>GGSKPDCTAAMRDVRQQYESVAAKNLQEAEEWYKSKFADLSEAANRNNDALRQAKQESTEYRRQVQSLTMEV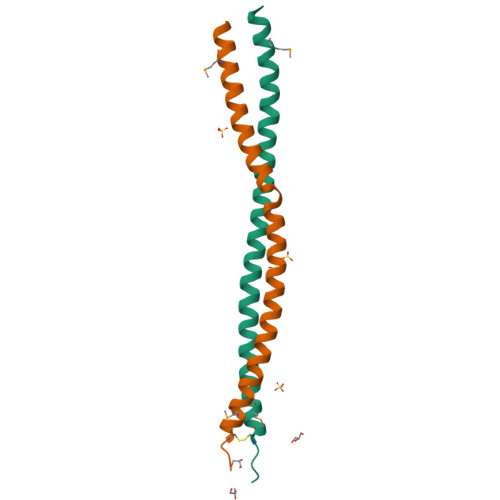DALKG[2x]>[2x]SGGAQLTTESMPFNVAEGKEVLLLVHNLPQQLFGYSWYKGERVD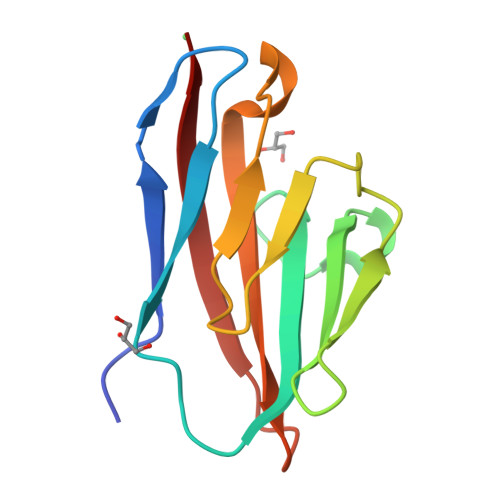GNRQIVGYAIGTQQATPGPANSGRETIYPNASLLIQNVTQNDTGFYTLQVIKSDLVNEEATGQFHVY>[2x]MPELPEVEAARRAIEENCLGKKIKRVIIADDNKVIHGISPSDFQTSILGKTIISARRKGKNLWLELDSPPFPSFQFGMAGAIYIKGVAVTKYKRSAVKDSEEWPSKYSKFFVELDDGLELSFTDKRRFAKVRLLANPTSVSPISELGPDALLEPMTVDEFAESLAKKKITIKPLLLDQGYISGIGNWIADEVLYQARIHPLQTASS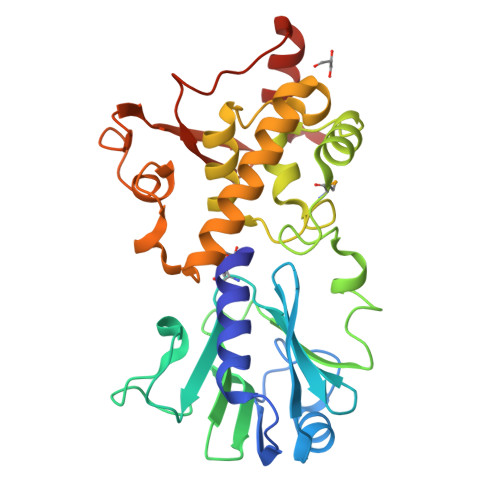LSKEQCEALHTSIKEVIEKAVEVDADSSQFPSNWIFHNREKKPGKAFVDGKKIDFITAGGRTTAYVPELQKLYGKCVDKLAAALEHHHHHH FcμR is the IgM antibody isotype-specific Fc receptor involved in the survival and activation of B cells. In this study, we image a complex of the ectodomain of human FcμR and the IgM-Fc pentameric core using single-particle cryogenic electron microscopy (cryo-EM). The analysis reveals multiple binding sites for the N-terminal Ig domain of FcμR on the Cμ4 domain dimers within the IgM constant region and provides a framework for understanding FcμR’s role in immunoglobulin recognition and signalling. A key common feature of the FcμR binding sites is that only the Cμ4 domains are involved in the interactions.

We resolved only the Ig domain of FcμR with the remaining ectodomain density appearing disordered at locations distal to the IgM binding site. Fig. 1a-b demonstrates the overall architecture of the multivalent engagement of the IgM pentamer by FcμR molecules. Each FcμR is similarly positioned relative to the IgM subunit. An IgM pentamer has ten potential FcμR binding sites, but only eight are found to be occupied.The two FcμR-absent positions are the front of subunit Fcμ5 (position 5f) and the back of subunit Fcμ1 (position 1b) though extremely low occupancy at position 5f may be suggested by features near the noise level in unsharpened cryo-EM maps. The tip of the hairpin-1 region in the J chain may prevent the addition of an FcμR at position 5f by marginally blocking FcμR at Ser55-Thr57. Position 1b seems available for binding, but access to this site may be blocked by the hairpin-2 region in the J chain, a highly flexible loop containing 30 residues that remains unstructured in the cryo-EM map. The eight binding sites on IgM pentamer are not equally occupied by FcμR. The highest FcμR occupancies are at positions 1f and 3f (nearly 90%), followed by 2b-4b and 4f (40-60%), and with 2f and 5b the lowest (around 10%). The low occupancy at position 2f, which is sandwiched between the two most heavily occupied FcμR binding sites, may indicate a subtle steric hindrance between adjacent FcμR molecules. Multivalent engagement of IgM facilitates the capture of soluble IgM or IgM immune complexes by FcμR anchored on cell surfaces, leading to FcμR clustering and signalling.

>[10x]IAELPPKVSVFVPPRDGFFGNPRKSKLICQATGFSPRQIQVSWLREGKQVGSGVTTDQVQAEAKESGPTTYKVTSTLTIKESDWLGQSMFTCRVDHRGLTFQQNASSMCVPDQDTAIRVFAIPPSFASIFLTKSTKLTCLVTDLTTYDSVTISWTRQNGEAVKTHTNISESHPNATFSAVGEASICEDDWNSGERFTCTVTHTDLPSPLKQTISRPKGVALHRPDVYLLPPAREQLNLRESATITCLVTGFSPADVFVQWMQRGQPLSPEKYVTSAPMPEPQAPGRYFAHSILTVSEEEWNTGETYTCVVAHEALPNRVTERTVDKSTGKPTLYNVSLVMSDTAGTCY;>[8x]RILPEVKVEGELGGSVTIKCPLPEMHVRIYLCREMAGSGTCGTVVSTTNFIKAEYKGRVTLKQYPRKNLFLVEVTQLTESDSGVYACGAGMNTDRGKTQKVTLNVHSEYEPSWEEQPMPETPKWFHLPYLFQMPAYASSSKFVTRVTTPAQRGKVPPVHHSSPTTQITHRPRVSRASSVAGDKPRTFLPSTTASKISALEGLLKPQTPSYNHHTRLHRQRALDYGSQSGREGQG;> MKNHLLFWGVLAVFIKAVHVKAQEDERIVLVDNKCKCARITSRIIRSSEDPNEDIVERNIRIIVPLNNRENISDPTSPLRTRFVYHLSDLCKKCDPTEVELDNQIVTATQSNICDEDSATETCYTYDRNKCYTAVVPLVYGGETKMVETALTPDACYPD> GSHMNGEPDIAQLKGLSPSQRQAYAVQLKNRGNHFFTAKNFNEAIKYYQYAIELDPNEPVFYSNISACYISTGDLEKVIEFTTKALEIKPDHSKALLRRASANESLGNFTDAMFDLSVLSLNGDFDGASIEPMLERNLNKQAMKVLNENLSKDEGRGSQVLPSNTSLASFFGIFDSHLEVSSVNTSSNYDTAYALLSDALQRLYSATDEGYLVANDLLTKSTDMYHSLLSANTVDDPLRENAALALCYTGIFHFLKNNLLDAQVLLQESINLHPTPNSYIFLALTLADKENSQEFFKFFQKAVDLNPEYPPTYYHRGQMYFILQDYKNAKEDFQKAQSLNPENVYPYIQLACLLYKQGKFTESEAFFNETKLKFPTLPEVPTFFAEILTDRGDFDTAIKQYDIAKRLEEVQEKIHVGIGPLIGKATILARQSSQDPTQLDEEKFNAAIKLLTKACELDPRS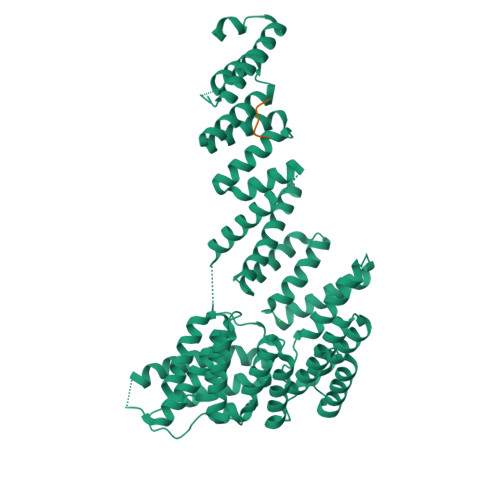EQAKIGLAQLKLQMEKIDEAIELFEDSAILARTMDEKLQATTFAEAAKIQKRLRADPIISAKMELTLARYRAKGML;> EVPADTEMEEVD> MQIGFNFTLTGTLDMVQQMIKERKIDYVEMLIDNFVHLPPEQIADSFDCPVAFHIMLSKYLERDREALAALGKRLRRFIDVMRPVYVS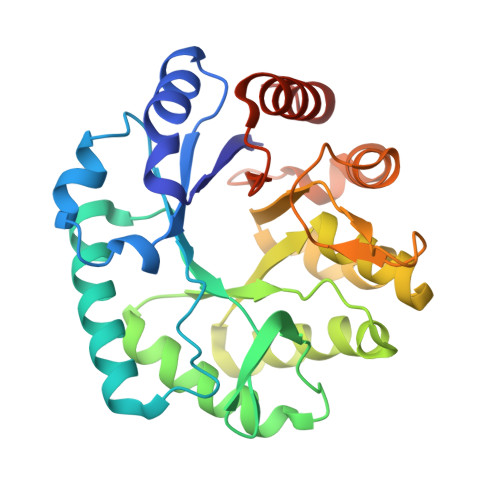DHILYFTHNGRSLFHLGEIDYGEYDHVRSKVEQWQDMLGTRLYLENYPSIMDGAWDAPSFYERLSRETGVGVLFDASNAICAQNNTGAPVELWKKIIETTRHFHVAGYGTAFIEPRVKADTSDREMAEDTLDFLSRMRTSFDKPGATITYERDFDIDYESISVDLKRLRDIFPCVEEERH> MPVLNLNDPQAVERYEEFMRQSPYGQVTQDLGWAKVKNNWEPVDVYLEDDQGAIIAAMSMLLGDTPTDKKFAYASKGPVMDVTDVDLLDRLVDEAVKALDGRAYVLRFDPEVAYSDEFNTTLQDHGYVTRNRNVADA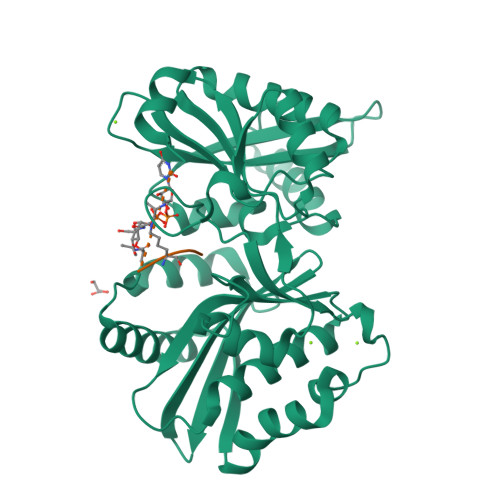GMHATIQPRLNMVLDLTKFPDAKTTLDLYPSKTKSKIKRPFRDGVEVHSGNSATELDEFFKTYTTMAERHGITHRPIEYFQRMQAAFDADTMRIFVAEREGKLLSTGIALKYGRKIWYMYAGSMDGNTYYAPYAVQSEMIQWALDTNTDLYDLGGIESESTDDSLYVFKHVFVKDAPREYIGEIDKVLDPEVYAELVKD;> AEKAA> GKSTTLFSRHTKAIVWGMQTRAVQGMLDFDYVCSRDEPSVAAMVYPFTGDHKQKFYWGHKEILIPVFKNMADAMRKHPEVDVLINFASLRSAYDSTMETMNYAQIRTIAIIAEGIPEALTRKLIKKADQKGVTIIGPATVGGIKPGCFKIGNTGGMLDNILASKLYRPGSVAYVSRSGGMSNELNNIISRTTDGVYEGVAIGGDR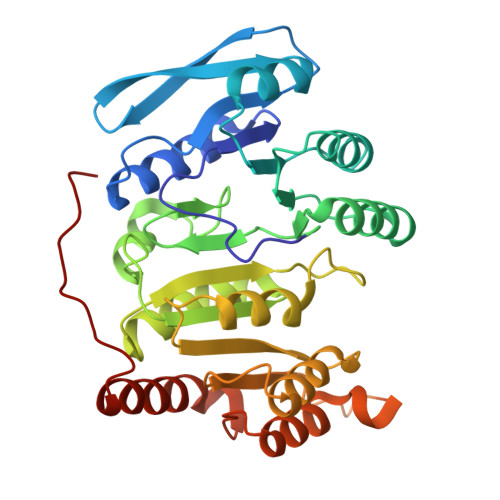YPGSTFMDHVLRYQDTPGVKMIVVLGEIGGTEEYKICRGIKEGRLTKPIVCWCIGTCATMFSSEVQFGHAGACANQASETAVAKNQALKEAGVFVPRSFDELGEIIQSVYEDLVANGVIVPAQEVPPPTV>[2x]MAHHHHHHVGTFENITAAPADPILGLADLFR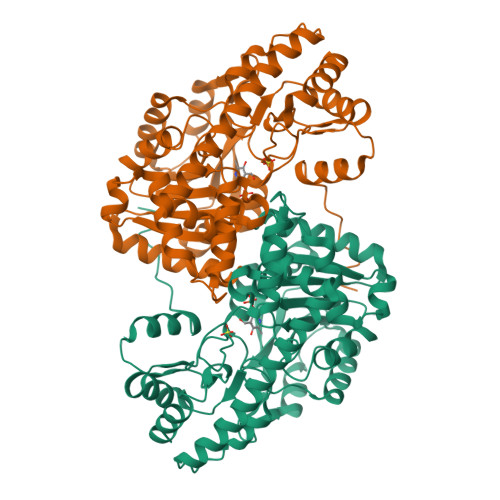ADERPGKINLGIGVYFDETGKIPVLTSVKKAEQYLLENETTKTYLGIDGIPEFGRCTQELLFGKGSALINDKRARTAQTPGGTGALRVAADFLAKNTSVKRVWVSNPSWPNHKSVFNSAGLEVREYAYYDAENHTLDFDALINSLNEAQAGDVVLFHGCCHNPTGIDPTLEQWQTLAQLSVEKGWLPLFDFAYQGFARGLEEDAEGLRAFAAMHKELIVASSYSKNFGLYNERVGACTLVAADSETVDRAFSQMKAAIRANYSNPPAHGASVVATILSNDALRAIWEQELTDMRQRIQRMRQLFVNTLQEKGANRDFSFIIKQNGMFSFSGLTKEQVLRLREEFGVYAVASGRVNVAGMTPDNMAPLCEAIVAVL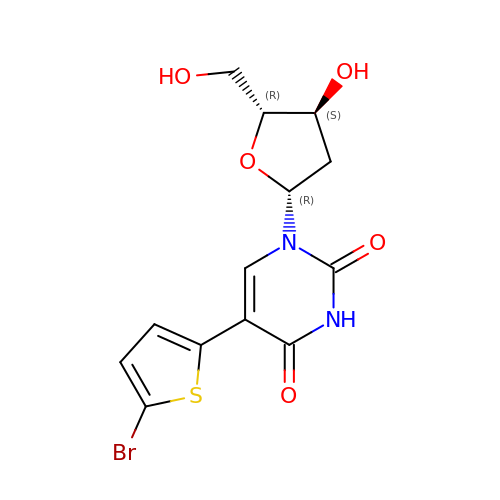5-BROMOTHIENYLDEOXYURIDINE | C13 H13 Br N2 O5 S | IGUZFFOBAZCVRK-VAOFZXAKSA-N> RDENKLEELKEQGFARIAIANEPPFTAVGADGKVSGAAPDVAREIFKRLGVADVVASISEYGAMIPGLQAGRHDAITAGLFMKPERCAAVAYSQPILCDAEAFALKKGNPLGLKSYKDIADNPDAKIGAPGGGTEEKLALEAGVPRDRVIVVPDGQSGLKMLQDGRIDVYSLPVL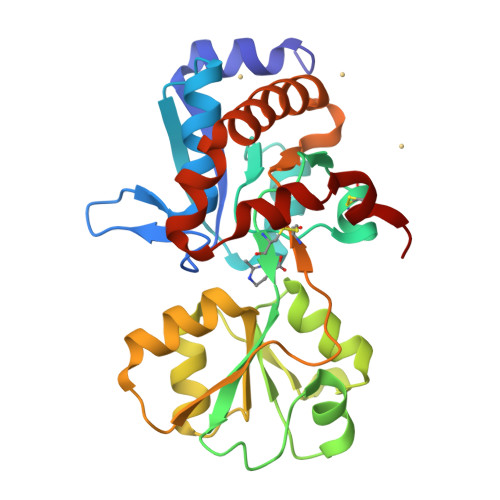SINDLVSKANDPNVEVLAPVEGAPVYCDGAAFRKGDEALRDAFDVELAKLKESGEFAKIIEPYGFSAKAAMSTTREKLCAAK> SHMREESLQLMDLLGLERSAWGNIPLMRKAYLKKCKEFHPDKGGDEEKMKKMNTLYKKMEDGVKYAHQPDFGGFWDATEIPTYGTDEWEQWWNAFNEENLFCSEEMPSSDDEAT;> MNTIQQLMMILNSASDQPSENLISYFNNCTVNPKESILKRVKDIGYIFKEKFAKA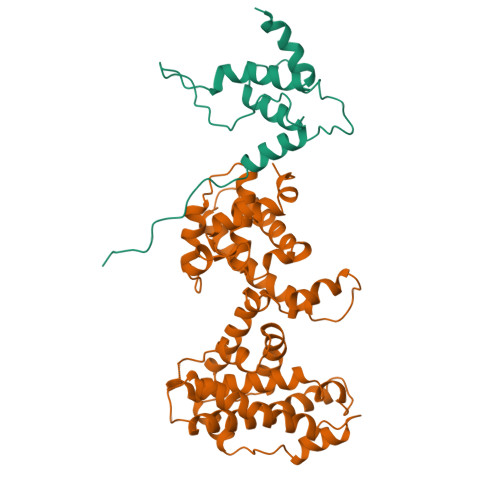VGAGCVAIGSQRYKLGVRLYYRVMESMLKSEEERLSIQNFSKLLNDNIFHMSLLACALEVVMATYSRSTSQNLDSGTDLSFPWILNVLNLKAFDFYKVIESFIKAEGNLTREMIKHLERCEHRIMESLAWLSDSPLFDLIKQSKLVPRGSTSLSLFYKKVYRLAYLRLNTLCERLLSEHPELEHIIWTLFQHTLQNEYELMRDRHLDQIMMCSMYGICKVKNIDLKFKIIVTAYKDLPHAVQETFKRVLIKEEEYDSIIVFYNSVFMQRLKTNILQYA> MPIRSISNTFNRGELDPTLFARDDLDIYDKGARKLRNMIALWTGAARIAPGTIYIDMMVDRENGNAVIQDPLMVKGFDFTYDADAEITYTIIIRKSGTNIAFDIYYADTLQTTVTSTAYLATQIQDIHVAAAHDRVLILHENVQIRQLKRGASHSSWSLTTFNPRVYPTYDFSVIGEAINYQSFTFTLSATTGSITIT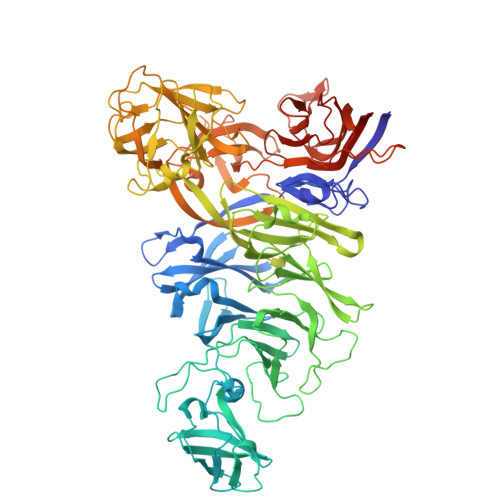SSSAVFTHNHVGGLFRSLGGTARITAVASTTSASATVLDNFTGTSCAGNLSSLAEKLWNSDTTTAPVSANRGWPARGVFYLNRLILGRSLAVKNLVNLSTAGVYDNFDDADLDGLVAFSVTFNGKGEQSVQSIVADDSILFTTANKLFAQSPLVESPITINNVYFAPQSQSPATSIEAASIDNQTLFVSSDRTKVMQAMYSTADGKYITLPATMLSNSIVDYINSNGTWEPAGISTRLYLATQDNGTMLLYSTLQTQNVAGWSLRTTTGKFRQVIGEGRQSHVIVEREINIGASFEQTLDYAYLSDPTFKARYDVTEFFASSPMTSAIGVLENQNDYILIGNQAPFTALDIDFNLVASSDCQLQFEYLDGNGFWDVFTPTDNTSGFTVDGTITWTFDDVLNWAPYQVNAIENQYWIRIKRLAETVNTAPVIGQVLINTGNRIYLERQSFDEYMDSTQIVTSDSNGLVTGLTHLAGQQVYAITEDGATIGSSFVDASGETSVKNVNTTLTVGMQYKPELIPMPLYAPTQMGDSLYAEKYVQDLYVDYVDSLYLQAGFRPQLTDIPNMHLGNYTLGQSVPPQTGIYRICPRGDWEPRQEFVITQSQPGPMTIIGVGYNVEVA> SIIQFLQRPVLIDNIEIVAGTTADNNTALSRYVLDRTNPQKYIKQWTLPSTVLK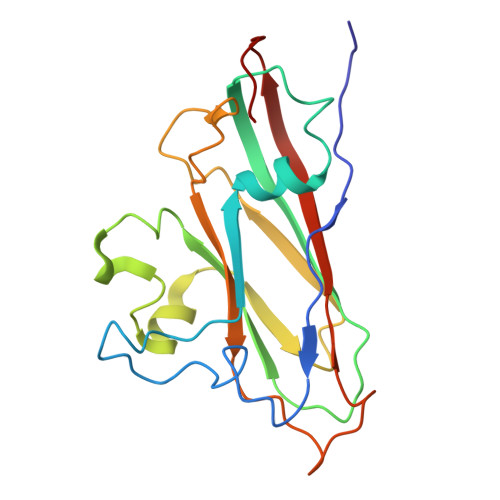AGGKAQKLANFKYLRCDVQVKIVLNANPFIAGRLYLAYSPYDDKVAPERRIIYTSRAGVTGYPGVELDFQLDNSVEMTIPYASFQEAYDLVSGNEDFVQLYLFTIAPVLGPSAESANSKVDLSVYMWLDNISLVIPTYRLNP> GLPTMNTPGSNQFLTSDDFQSPSAMPQFDVTPEMHIPGEVRNLMEIAEVDSVMPINNDSAAKVSSMEAYRVELSTNTNAGTQVFGFQ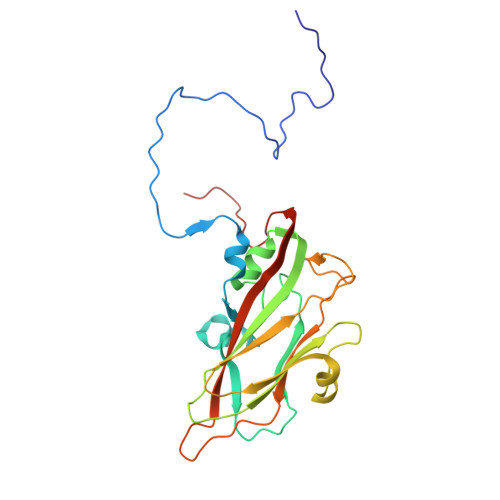LNPGAESVMNRTLMGEILNYYAHWSGSIKITFVFCGSAMTTGKFLLSYAPPGAGAPKTRKDAMLGTHVVWDVGLQSSCVLCIPWISQTHYRFVEKDPYTNAGFVTCWYQTSVVSPASNQPKCYMMCMVSACNDFSVRMLRDTKFIEQTSFYQ>MQISSDYIPDSKFYKVEAIVRPWRIQQVSSALLKIGIRGVTVSDVRGFGAQGGSTERHGGSEFSEDKFVAKVKMEIVVKKDQVESVINTIIEGARTGEIGDGKIFVLPVSDVIRVRTGERGEKAEKMTGDML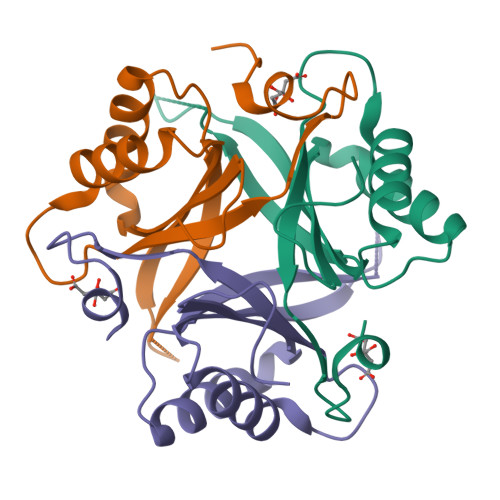SPS[3x]>ENLMQVYQQARLSNPELRKSAADRDAAFEKINEARSPLLPQLGLGADYTYSNGYRDANGINSNETSASLQLTQTLFDMSKWRGLTLQEKAAGIQDVTYQTDQQTLILNTANAYFKVLNAIDVLSYTQAQKEAIYRQLDQTTQRFNVGLVAITDVQNARAQYDTVLANEVTARNNLDNAVEELRQVTGNYYPELASLNVEHFKTDKPKAVNALLKEAENRNLSLLQARLSQDLAREQIRQAQDGHLPTLNLTASTGISDTSYSGSKTNSTQYDDSNMGQNKIGLNFSLPLYQGGMVNSQVKQAQYNFVGASEQLESAHRSVVQTVRSSFNNINASISSINAYKQAVVSAQSSLDAMEAGYSVGTRTIVDVLDATTTLYDAKQQLANARYTYLINQLNIKYALGTLNEQDLLALNSTLGKPIPTSPESVAPETPDQDAAADGYNAHSAAPAVQ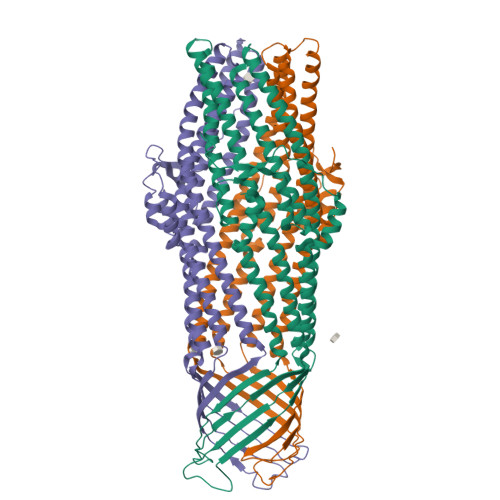PTAARANSNNGNPFRH[3x]> MGSDKIHHHHHHENLYFQGMNLVQDKVTIITGGTRGIGFAAAKIFIDNGAKVSIFGETQEEVDTALAQLKELYPEEEVLGFAPDLTSRDAVMAAVGQVAQKYGRLDVMINNAGITSNNVFSRVSEEEFKHIMDINVT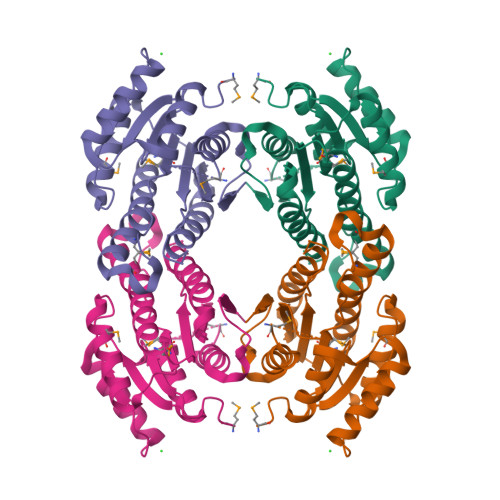GVFNGAWCAYQCMKDAKKGVIINTASVTGIFGSLSGVGYPASKASVIGLTHGLGREIIRKNIRVVGVAPGVVNTDMTNGNPPEIMEGYLKALPMKRMLEPEEIANVYLFLASDLASGITATTVSVDGAYRP>[2x]MKIGSGEKLLFIGDSITDCGRARPEGEGSFG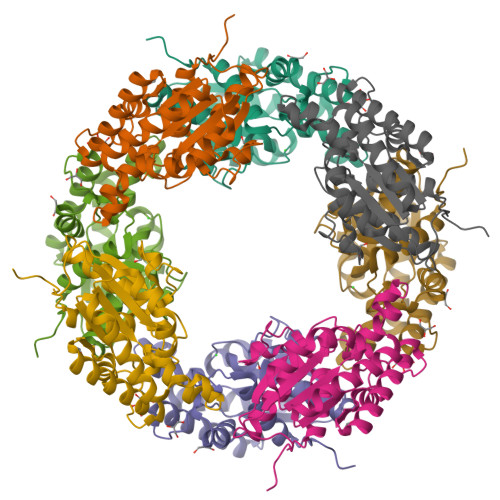ALGTGYVAYVVGLLQAVYPELGIAVVNKGISGNTVRDLKARWEEDVIAQKPDWVSIMIGINDVWRQYDLPFMKEKHVYLDEYEATLRSLVLETKPLVKGIILMTPFYIEGNEQDPMRRTMDQYGRVVKQIAEETNSLFVDTQAAFNEVLKTLYPAALAWDRVHPSVAGHMILARAFLREIGFEWVRSR>MSSSTDNFSATMRDGLSNLARRLRFAMKEGSIWLGEQRMILLHTAALGALRKELVDTLGMERARGLFMRMGFHSGVRDAELAKTMRSGHSDFGMLEMGPCLHTIEGVVRVTPLTVDINIAAGVYHGEFLWEDSFEGDVHRQMFGVAQAPVCWMQIGYATGYTSALMGKTILYRELECVGCGHPHCRILGKPLEQWEDGEA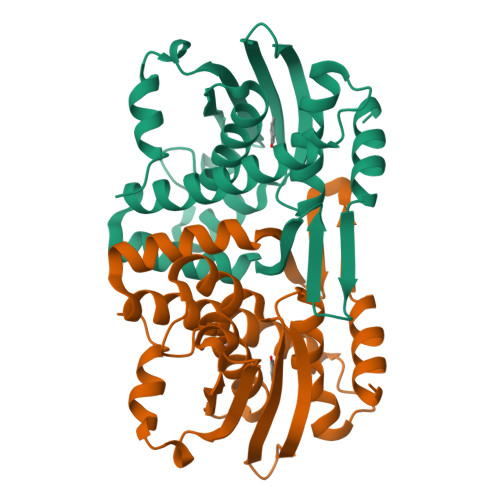ELALYQPDPVI[2x]> MSQEALKAPVVVLGAGLASVSFVAELRQAGYQGLITVVGDEAERPYDRPPLSKDFMAHGDAEKIRLDCKRAPEVEWLLGVTAQSFDPQAHTVALSDGRTLPYGTLVLATGAAPRALPTLQGATMPVHT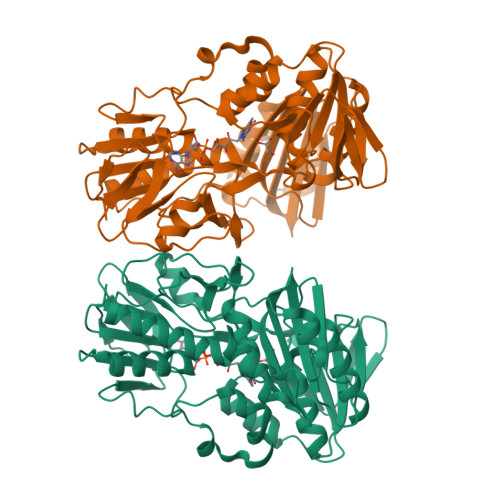LRTLEDARRIQAGLRPQSRLLIVGGGVIGLELAATARTAGVHVSLVETQPRLMSRAAPATLADFVARYHAAQGVDLRFERSVTGSVDGVVLLDDGTRIAADMVVVGIGVLANDALARAAGLACDDGIFVDAYGRTTCPDVYALGDVTRQRNPLSGRFERIETWSNAQNQGIAVARHLVDPTAPGYAELPWYFSDQGALRIQVAGLASGDEEIVRGEVSLDAPKFTLIELQKGRIVGATCVNNARDFAPLRRLLAVGAKPDRAALADPATDLRKLAAAVAA> GSHMDTPSSPSIDQVEPYSSTAQVQFDEPEATGGVPILKYKAEWRAVGEEVWHSKWYDAKEASMEGIVTIVGLKPETTYAVRLAAL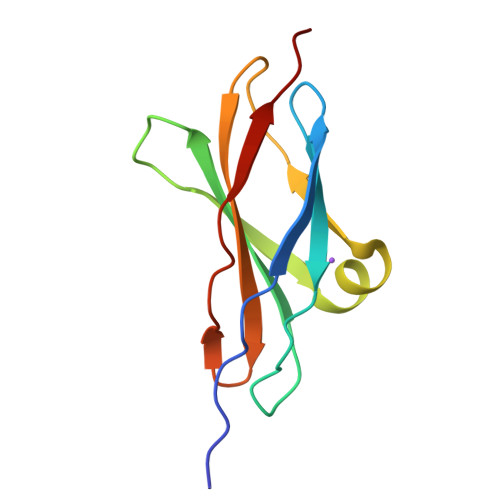NGKGLGEISAASEFKTQPV> GCCSHPACSVN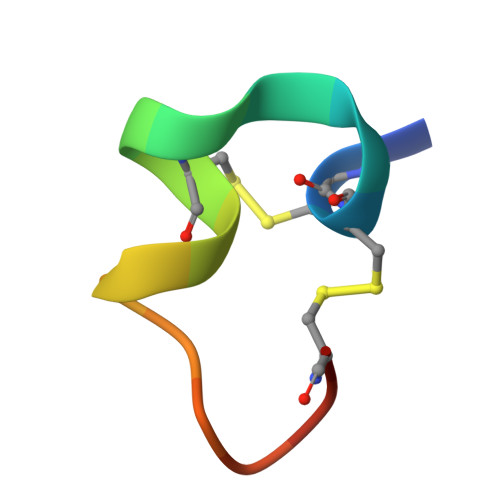HPELCX>ANSLVEEFKSGNIERECIEERCSKEEAREVFEDDEKTETFWNVYVDGDQCSSNPCHYRGICKDGIGSYTCTCLSGYEGKNCERVL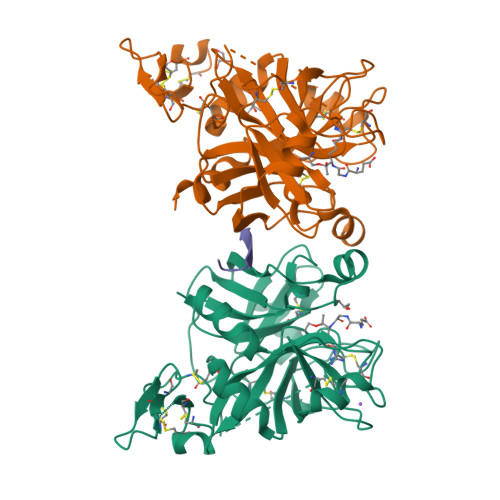YKSCRVDNGNCWHFCKHVQNDIQCSCAEGYLLGEDGHSCVAGGNFSCGRNIKTRNKREANLPDFVQSQNATLLKKSDNPSPDIRIVNGMDCKLGECPWQAALVDEKEGVFCGGTILSPIYVLTAAHCINETETISVVVGEIDKSRIETGPLLSVDKIYVHKKFVPPQKAYKFDLAAYDYDIAIIQMKTPIQFSENVVPACLPTADFANQVLMKQDFGIVSGFGRIVEKGPKSKTLKVLKVPYVDRHTCMVSSETPITPNMFCAGYDTLPRDACQGDSGGPHTTVYRDTHFITGIVSSGEGCARNGKYGNYTKLSKFIPWIKRIMRQKLPSTESSTGRL[2x];> GNEEEEEDDGDIFADIFI In the periplasm, M is randomly epimerized to G or partially acetylated, and the mature alginate is directed to the transmembrane β-barrel protein AlgE in the outer membrane for conveyance to the extracellular space. Briefly, the structures include 18 antiparallel strands (S1–S18) that cross the membrane to varying degrees, nine extracellular loops (L1–L9) and eight periplasmic turns (T1–T8). The loops and turns range in size from two to 43 residues, with L1 coordinating a calcium ion. Both the N- and C-termini are in the periplasm. The cavity within the AlgE barrel has been proposed to act as a pore for alginate, a random, linear copolymer of 1,4-linked β-d-mannuronic acid (M) and its C-5 epimer α-l-guluronic acid (G).

The best crystals were obtained with 7.8 MAG at 20°C. These yielded three crystal forms in space groups C2, P212121, P21 that diffracted to 1.9, 2.4 and 2.8 Å resolution, respectively. In contrast, the asymmetric units of AlgE-2.4 and AlgE-2.8 contain two molecules (molecules A and B). For all in meso structures, type I packing was observed, as is the norm for crystals grown in a lipidic mesophase environment. Interestingly, we find that L2 and T8, while ordered in some crystal forms, are disordered in others. Disorder, where electron density is either not observed or is ill-defined in the map, suggests that the corresponding loops, or parts thereof, are flexible and, in certain cases, may have relocated to reside outside the barrel. In the case of AlgE-2.4, which has two molecules in the asymmetric unit, T8 is disordered in molecule A (AlgE-2.4A) and is ordered in molecule B (AlgE-2.4B). These two crystal forms are interpreted as examples of the alginate pore in which its periplasmic gate (P-­gate) is open and closed, respectively. It appears therefore that in this collection of six models we have an ensemble of structures that map a conformational landscape for alginate transport. We refer to this as the double-gate model.

>ANSGEAPKNFGLDVKITGESENDRDLGTAPGGTLNDIGIDLRPWAFGQWGDWSAYFMGQAVAATDTIETDTLQSDTDDGNNSRNDGREPDKSYLAAREFWVDYAGLTAYPGEHLRFGRQRLREDSGQWQDTNIEALNWSFETTLLNAHAGVAQRFSEYRTDLDELAPEDKDRTHVFGDISTQWAPHHRIGVRIHHADDSGHLRRPGEEVDNLDKTYTGQLTWLGIEATGDAYNYRSSMPLNYWASATWLTGDRDNLTTTTVDDRRIATGKQSGDVNAFGVDLGLRWNIDEQWKAGVGYARGSGGGKDGEEQFQQTGLESNRSNFTGTRSRVHRFGEAFRGELSNLQAATLFGSWQLREDYDASLVYHKFWRVDDDSDIGTSGINAALQPGEKDIGQELDLVVTKYFKQGLLPASMSQYVDEPSALIRFRGGLFKPGDAYGPGTDSTMHRAFVDFIWRF[2x]>[2x]MRRETVGEFSSDDDDDILLELGTRPPRFTQIPPSSAALQTQIPTTLEVTTTTLNNKQSKNDNQLVNQLNKAQGEASMLRDKINFLNIEREKEKNIQAVKVNELQVKHLQELAKLKQELQKLEDEKKFLQMEARGKSKREVITNVKPPSTTLSTNTNTITPDSSSVAIEAKPQSPQSKKRKISDNLLKKNMVPLNPNRIIPDETSLFLESILLHQIIGADLSTIEILNRLKLDYITEFKFKNFVIAKGAPIGKSIVSLLLRCKKTLTLDRFIDTLLEDIAVLIKEISVHPNESKLAVPFLVALMYQIVQFRPSATHNLALKDCFLFICDLIRIYHHVLKVPIHESNMNLHVEPQIFQYELIDYLIISYSFDLLEGILRVLQSHPKQTYMEFFDENILKSFEFVYKLALTISYKPMVNVIFSAVEVVNIITSIILNMDNSSDLKSLISGSWWRDCITRLYALLEKEIKSGDVYNENVDTTTLHMSKYHDFFGLIRNIGDNELGGLISKLIYTDRLQSVPRVISKEDIGMDSDKFTAPIIGYKMEKWLLKLKDEVLNIFENLLMIYGDDATIVNGEMLIHSSKFLSREQALMIERYVGQDSPNLDLRCHLIEHTLTIIYRLWKDHFKQLREEQIKQVESQLIMSLWRFLVCQTETVTANEREMRDHRHLVDSLHDLTIKDQASYYEDAFEDLPEYIEEELKMQLNKRTGRIMQVKYDEKFQEMARTILESKSFDLTTLEEADSLYISMGL;>MESHVKYLDELILAIKDLNSGVDSKVQIKKVPTDPSSSQEYAKSLKILNTLIRNLKDQRRNNIMKNDTIFSKTVSALALLLEYNPFLLVMKDSNGNFEIQRLIDDFLNISVLNYDNYHRIWFMRRKLGSWCKACVEFYGKPAKFQLTAHFENTMNLYEQALTEVLLGKTELLKFYDTLKGLYILLYWFTSEYSTFGNSIAFLDSSLGFTKFDFNFQRLIRIVLYVFDSCELAALEYAEIQLKYISLVVDYVCNRTISTALDAPALVCCEQLKFVLTTMHHFLDNKYGLLDNDPTMAKGILRLYSLCISNDFSKCFVDHFPIDQWADFSQSEHFPFTQLTNKALSIVYFDLKRRSLPVEALKYDNKFNIWVYQSEPDSSLKNVTSPFDDRYKQLEKLRLLVLKKFNKTERGTLLKYRVNQLSPGFFQRAGNDFKLILNEASVSIQTCFKTNNITRLTSWTVILGRLACLESEKFSGTLPNSTKDMDNWYVCHLCDIEKTGNPFVRINPNRPEAAGKSEIFRILHSNFLSHPNIDEFSESLLSGILFSLHRIFSHFQPPKLTDGNGQINKSFKLVQKCFMNSNRYLRLLSTRIIPLFNISDSHNSEDEHTATLIKFLQSQKLPVVKENLVIAWTQLTLTTSNDVFDTLLLKLIDIFNSDDYSLRIMMTLQIKNMAKILKKTPYQLLSPILPVLLRQLGKNLVERKVGFQNLIELLGYSSKTILDIFQRYIIPYAIIQYKSDVLSEIAKIMCDGDTSLINQMKVNLLKKNSRQIFAVALVKHGLFSLDILETLFLNRAPTFDKGYITAYLPDYKTLAEITKLYKNSVTKDASDSENANMILCSLRFLITNFEKDKRHGSKYKNINNWTDDQEQAFQKKLQDNILGIFQVFSSDIHDVEGRTTYYEKLRVINGISFLIIYAPKKSIISALAQISICLQTGLGLKEVRYEAFRCWHLLVRHLNDEELSTVIDSLIAFILQKWSEFNGKLRNIVYSILDTLIKEKSDLILKLKPYTTLALVGKPELGILARDGQFARMVNKIRSTTDLIPIFANNLKSSNKYVINQNLDDIEVYLRRKQTERSIDFTPKKVGQTSDITLVLGALLDTSHKFRNLDKDLCEKCAKCISMIGVLDVTKHEFKRTTYSENEVYDLNDSVQTIKFLIWVINDILVPAFWQSENPSKQLFVALVIQESLKYCGLSSESWDMNHKELYPNEAKLWEKFNSVSKTTIYPLLSSLYLAQSWKEYVPLKYPSNNFKEGYKIWVKRFTLDLLKTGTTENHPLHVFSSLIREDDGSLSNFLLPYISLDIIIKAEKGTPYADILNGIIIEFDSIFTCNLEGMNNLQVDSLRMCYESIFRVFEYCKKWATEFKQNYSKLHGTFIIKDTKTTNMLLRIDEFLRTTPSDLLAQRSLETDSFERSALYLEQCYRQNPHDKNQNGQLLKNLQITYEEIGDIDSLDGVLRTFATGNLVSKIEELQYSENWKLAQDCFNVLGKFSDDPKTTTRMLKSMYDHQLYSQIISNSSFHSSDGKISLSPDVKEWYSIGLEAANLEGNVQTLKNWVEQIESLRNIDDREVLLQYNIAKALIAISNEDPLRTQKYIHNSFRLIGTNFITSSKETTLLKKQNLLMKLHSLYDLSFLSSAKDKFEYKSNTTILDYRMERIGADFVPNHYILSMRKSFDQLKMNEQADADLGKTFFTLAQLARNNARLDIASESLMHCLERRLPQAELEFAEILWKQGENDRALKIVQEIHEKYQENSSVNARDRAAVLLKFTEWLDLSNNSASEQIIKQYQDIFQIDSKWDKPYYSIGLYYSRLLERKKAEGYITNGRFEYRAISYFLLAFEKNTAKVRENLPKVITFWLDIAAASISEAPGNRKEMLSKATEDICSHVEEALQHCPTYIWYFVLTQLLSRLLHSHQSSAQIIMHILLSLAVEYPSHILWYITALVNSNSSKRVLRGKHILEKYRQHSQNPHDLVSSALDLTKALTRVCLQDVKSITSRSGKSLEKDFKFDMNVAPSAMVVPVRKNLDIISPLESNSMRGYQPFRPVVSIIRFGSSYKVFSSLKKPKQLNIIGSDGNIYGIMCKKEDVRQDNQYMQFATTMDFLLSKDIASRKRSLGINIYSVLSLREDCGILEMVPNVVTLRSILSTKYESLKIKYSLKSLHDRWQHTAVDGKLEFYMEQVDKFPPILYQWFLENFPDPINWFNARNTYARSYAVMAMVGHILGLGDRHCENILLDIQTGKVLHVDFDCLFEKGKRLPVPEIVPFRLTPNLLDALGIIGTEGTFKKSSEVTLALMRKNEVALMNVIETIMYDRNMDHSIQKALKVLRNKIRGIDPQDGLVLSVAGQTETLIQEATSEDNLSKMYIGWLPFW[2x]

The ataxia-telangiectasia mutated (ATM) and ATM-Rad3-related (ATR) are apical kinases that orchestrate the multifaceted DNA damage response to a variety of insults and regulate genomic stability. The basal kinase activity of ATR plays critical regulatory roles during normal cell-cycle progression and aberrant activation of ATR signaling pathway can drive cells into senescence. In short, our study reveals a novel gating mechanism by which kinase N-lobe toggles between two alternative docking sites and recurrently commits the Mec1/ATR kinase for substrate recruitment, confined catalysis and product release.

We next determined the structure of Mec1-Ddc2 complex endogenously activated by MMS. Only one state could be stably classified with a resolution of 4.0 Å. The assembly adopts an asymmetric conformation despite having two identical Mec1-Ddc2 heterodimers. The whole molecule is significantly compressed, with the length and height have been reduced to 200 Å and 155 Å, respectively. We refer two monomers as ‘MMS-mono1’ and ‘MMS-mono2’, which demonstrate similar conformational changes at the domain level. After the Pincer and C-lobe are superimposed with each other, the FAT and kinase N-lobe move down by ~10 Å, whereas the Spiral of α-solenoid moves upwards by ~11 Å relative to their positions in the structure with the basal activity. The structures of Ddc2 and Mec1 Spiral domain are well matched, but the conformations of Bridge and FATKIN are significantly different, especially the significant displacement of LBE. FATC rotates 110 degrees downward, coupled with the displacement of PRD Kα10 along with Kα9 and Kα8 downward to the left in the range of 8~12 Å, which more significantly exposes the activation loop to facilitate substrate binding and catalysis. The most significant conformational divergence between the two monomers is at the position of LBE Kα4a and kinase N-lobe. In MMS-mono, the kinase N-lobe packs against the HEAT 25 R/26 R (residues 1005–1090), in close proximity to the Ser1333 residue in human ATR (corresponding to Thr1092 in Mec1).>[4x]M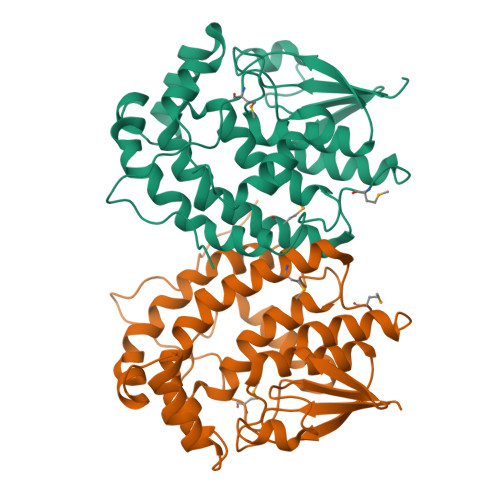ARNNTITLYDLQLESGCTISPYVWRTKYALKHKGFDIDIVPGGFTGILERTGGRSERVPVIVDDGEWVLDSWVIAEYLDEKYPDRPMLFEGPTQKNLMKFLDNWLWSTAVGPWFRCYILDYHDLSLPQDRDYVRWSREQWFLGGQRLEDVQAGREDRLPLVPPTLEPFRRILAETKWLGGDQPNFADYSALAVFLWTASVARTPPLTEDDPLRDWLDRGFDLFDGLGRHPGMNPLFGLKLREGDPEPFVRQTGPAGAGGQALNKGPQTTKMPPRVAEKAD>[4x]MQWSGARALEALLTVAGELRGPPLQLDTGQLLKIAKRGGVTAVEAVHAWRNALTGAPLNLTPEQVVAIASHDGGKQALETVQRLLPVLCQAHGLTPQQVVAIASHDGGKQALETVQRLLPVLCQAHGLTPEQVVAIASHDGGK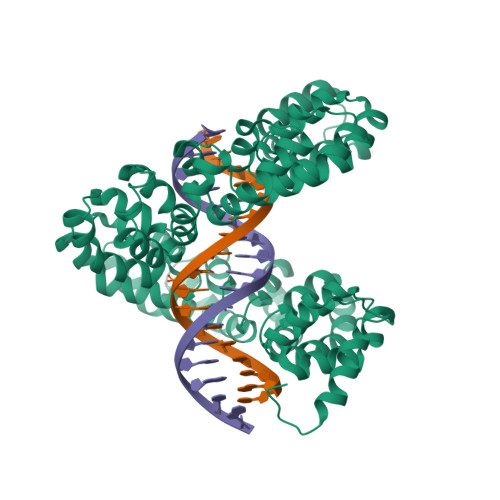QALETVQALLPVLCQAHGLTPEQVVAIASNGGGKQALETVQRLLPVLCQAHGLTPQQVVAIASNGGGKQALETVQRLLPVLCQAHGLTPQQVVAIASQGGKQALETVQRLLPVLCQAHGLTPQQVVAIASNNGGKQALETVQRLLPVLCQAHGLTPQQVVAIASHDGGKQALETVQRLLPVLCQAHGLTPQQVVAIASNNGGKQALETVQRLLPVLCQAHGLTPEQVVAIASNGGGKQALETVQRLLPVLCQAHGLTPEQVVAIASHDGGKQALETVQRLLPVLCQAHGLTPQQVVAIASNGGGRPALESIVAQLSRPDPALAALTNDHLVALACLGGRPALDAVKKLEHHHHHH> GPLGSSHEQFRAALQAVVDPGDPRSYLDNFIKIGEGSTGIVCIATVRSSGKLVAVKKMDLRKQQRRELLFNEVVIMRDYQHENVVEMYNSYLVGDELWVVMEFLEGGALTDIVTHTRMNEEQIAAVCLAVLQALSVLHAQGVIHRDIKSDSILLTHDGRVKLSDFGFCAQVSKEVPRRKSLVGTPYWMAPELISRLPYGPEVDIWSLGIMVIEMVDGEPPYFNEPPLK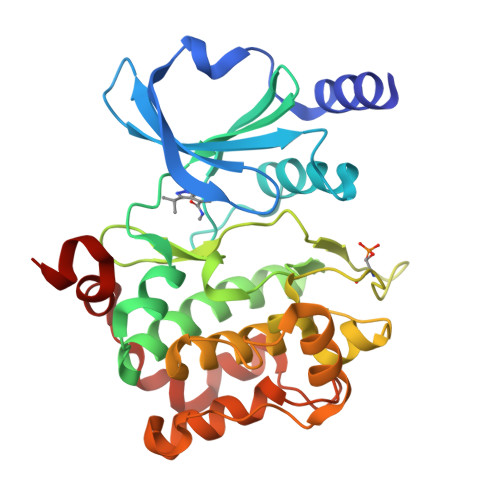AMKMIRDNLPPRLKNLHKVSPSLKGFLDRLLVRDPAQRATAAELLKHPFLAKAGPPASIVPLMRQNRTR>[2x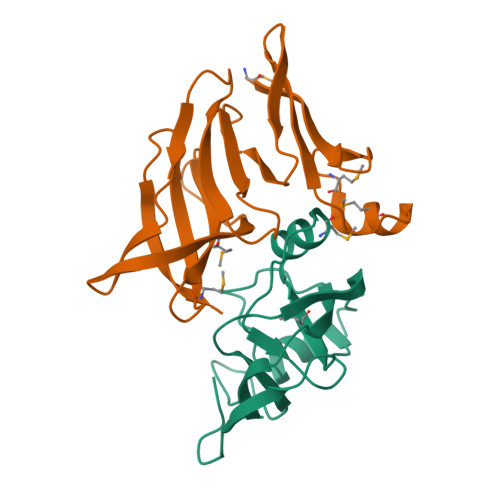]MGSSHHHHHHSQDPNSAWLEGTQVKTEIVPPGRQYQMVVAKGQAEAIMQGKPAFGGFAAPEPIPSQAYARDKLVILDRFKTDVSHVITVETTAPQKIHSGITGPLENYKGGVQQVEFVGDRNLKIVGTPGVLPVE;>[2x]MISDFERIREDGKVIDENMTVDQMIALGWSPCRVVEARWRWQEQLLSVVNSRGLLAIVVPDRQHLAILWNDDDTGVAATLYVVSGDRQQQIRIADQLLINGQLEAGIYSWFEQFPQVSPSIFTCMFSRQRDQAMFRVDIDASTGDIVSIQHSR> MRPEVEQELAHTLLVELLAYQFASPVRWIETQDVFLAEQMAERIVEIGPADTLSVMAKRTLASKYEAYDAAKSAQRQILCYSKDAKEIYYDVDPIEEEPEPAPAQAATPTAPAAPAATPAAAPAPVAAPPPPGVGPAAQVPDAPVTALEIVRALIAQKLKKPYQEVPLSKAIKDLVGGKSTLQNEILGDLGKEFGSTPEKPEDTPLDELGAAMQATFDGNLGKTSQGLIARLISSKMPGGFNITTARKYLETRWGLGPGRQDGVLLLAITMEPPSRLGSEADAKAFLDDVSQKYAANAGISLSTAAAAGPAAGAGGGMLMDPAALEALTSDQKALFKQQLELIARYLKLDIRAGDKAYQASQESAKVLQSQLDLWLAEHGDFYASGIEPVFSPLKARVYDSSWNWARQDALSMYYDIIFGRLKTVDREIVSQCIRIMNRANPTLLEFMQYHIDNCPTDRGETYQLAKELGAQLIENCKEVLNANPVYKDVAIPTGPKTTIDARGNLKYEEVPRPSCRKLEHYVQQMAAGGKISEYGNRIKVQNDLAKIYKLIKQQHKLPKTSQLEIKALYSDIIRALQMNENQILGQTNGKSLGLPKKGKPKAKTETIPFLHLRKKSVMGWEYNKKLTSLYLDCLEKAARDGLTFAGKYALMTGAGAGSIGAEVLQGLISGGAHVIVTTSRYSREVTEYYQSMYSRYGARGSQLVVVPFNQGSVQDVNALVEYIYDTKNGLGWDLDYIVPFAAISEQGRQIDGIDSKSELAHRIMLTNLIRLLGAVKTQKASRGYETRPAQVILPLSPNHGTFGSDGLYSESKLGLETLFNRWESENWSNYLTICGAIIGWTRGTGLMSGNNIVAEAVEKFGVRTFSQQEMAFNLLGLMAPTIVDLCQNEPVCADLNGGLQFIPNLNELMTRERKNLTETSEIRQAVTKETAAEN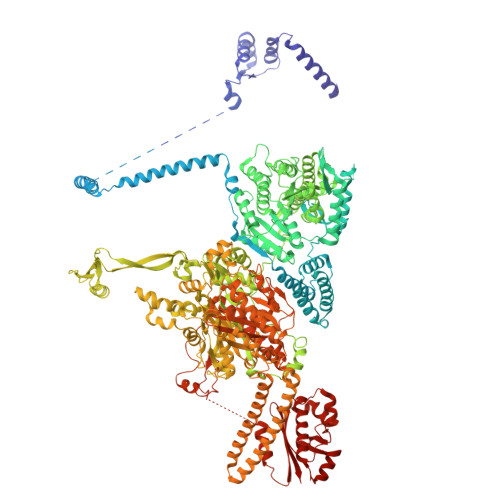KVVNGEASEALYKKKIIERRANIKFDFPPLPDWKKDIQPLNDKLKGMVDLEKVIVVTGFAEVGPWGNSRTRWEMEAYGEFSLEGCIEMAWIMGLIKNYNGLIKGKPYSGWVDAKTGEPVDDKDVKPKYEKYILEHSGIRLIEPELFGGYDPNKKQLLHEVVIQEDLDPFQCSAETAEQFKREHGDKVEIFEIPESGEYTVRFKKGATLWIPKALRFDRLVAGQIPTGWDAKRYGIPDDIIQQVDPVCLFVLVSTVEALLSSGITDPYEFYKYVHVSELGNCIGSGMGGATALRGMHRDRFLDKPLQNDILQESFINTMSAWVNMLLLSSSGPIKTPVAACATAVESVDVGVETILEGKARICLVGGFDDFGEEGSYEFANMKATSNAVDEFAHGRTPQEMSRPTTTTRNGFMESQGSGVQVIMTAKLALEMGVPIYGILALTTTASDKIGRSVPAPGQGVLTTAREHRGKFPSPLLDINYRRRQIERRTKQVMEEKEAEFEYLAAEIEALKAEGRPQSEIEEYAAHRAAHIEKTAEKQAKEILRSFGNFFWKNDPTIAPLRGALAVWGLTIDDLDVASFHGTSTKANDKNESSVICQQLAHLGRKKGNAVLGIFQKYLTGHPKGAAGAWMLNGCLQVLNTGLVPGNRNADNVDKVMEQFDYIVYPNRSIQTDGIKAFSVTSFGFGQKGAQCIGVHPKYLYATLDEQTYNEYCTKVQARQKKAYRYFHNGLINNTLFQAKEKAPYTDEQLSAVLLNPDARVVEDKKTGQLIFPPNFMKLSEKTQAAAQPKVSLESVLSREARRLESVNTRVGVDVEDISAINTDNDTFLDRNFTEAEQKYCLASKSGRSPQKAFAGRWTAKEAVFKALGVSSKGAGAALKDIEILVDENGAPTVSLHGAAAEAAKKAGIKSVSVSISYTDSQAAAIATAQL>[2x]MTNIRVAIVGYGNLGRSVEKLIAKQPDMDLVGIFSRRATLDTKTPVFDVADVDKHADDV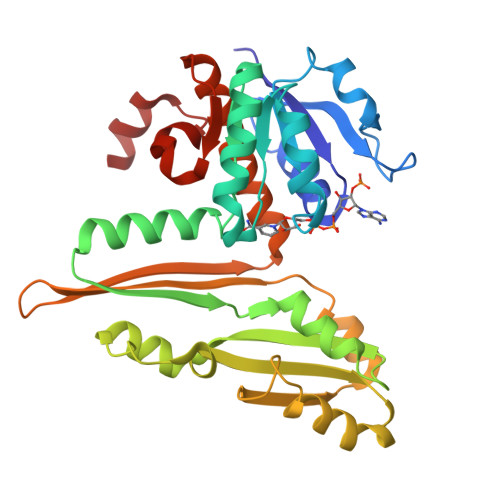DVLFLCMGSATDIPEQAPKFAQFACTVDTYDNHRDIPRHRQVMNEAATAAGNVALVSTGWDPGMFSINRVYAAAVLAEHQQHTFWGPGLSQGHSDALRRIPGVQKAVQYTLPSEDALEKARRGEAGDLTGKQTHKRQCFVVADAADHERIENDIRTMPDYFVGYEVEVNFIDEATFDSEHTGMPHGGHVITTGDTGGFNHTVEYILKLDRNPDFTASSQIAFGRAAHRMKQQGQSGAFTVLEVAPYLLSPENLDDLIARDV> GSMASLPVLQKESVFQSGAHAYRIPALLYLPGQQSLLAFAEQRAS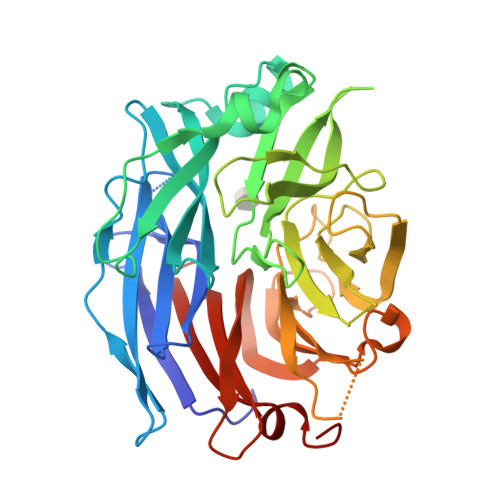KKDEHAELIVLRRGDYDAPTHQVQWQAQEVVAQARLDGHRSMNPCPLYDAQTGTLFLFFIAIPGQVTEQQQLQTRANVTRLCQVTSTDHGRTWSSPRDLTDAAIGPAYREWSTFAVGPGHCLQLNDRARSLVVPAYAYRKLHPIQRPIPSAFCFLSHDHGRTWARGHFVAQDTLECQVAEVETGEQRVVTLNARSHLRARVQAQSTNDGLDFQESQLVKKLVEPPPQGCQGSVISFPSPRSGPGSPAQWLLYTHPTHSWQRADLGAYLNPRPPAPEAWSEPVLLAKGSCAYSDLQSMGTGPDGSPLFGCLYEANDYEEIVFLMFTLKQAFPAEYLPQ N-(6-{4-[(4'-chlorobiphenyl-2-yl)methyl]piperazin-1-yl}-1,1-dioxido-1,2-benzothiazol-3-yl)-4-{[(2R)-4-(dimethylamino)-1-(phenylsulfanyl)butan-2-yl]amino}-3-nitrobenzenesulfonamide 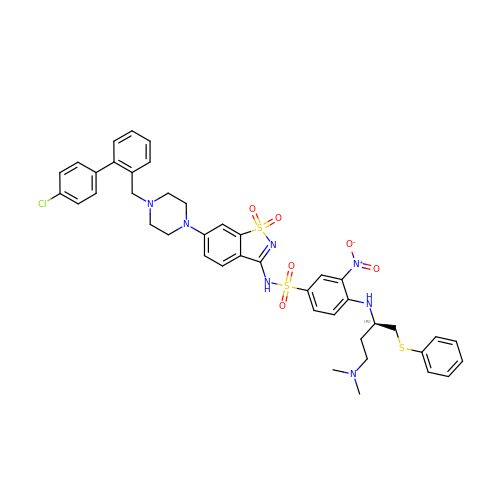| C42 H44 Cl N7 O6 S3 | IXACTXFUQMBZJI-MGBGTMOVSA-N> GAHMSGRGSSTDSMFSRFLPEKTDLKDYALPNASWCSDMLSLYQEFLEKTKSSGWIKLPSFKSNRDHIRGLKLPSGLAVSSDKGDCRIFTRCIQVEGQGFEYVIFFQPTQKKSVCLFQPGSYLEGPPGFAHGGSLAAMMDETFSKTAFLAGEGLFTLSLNIRFKNLIPVDSLVVMDVEVDKIEDQKLYMSCIAHSRDQQTVYAKSSGVFLQLQ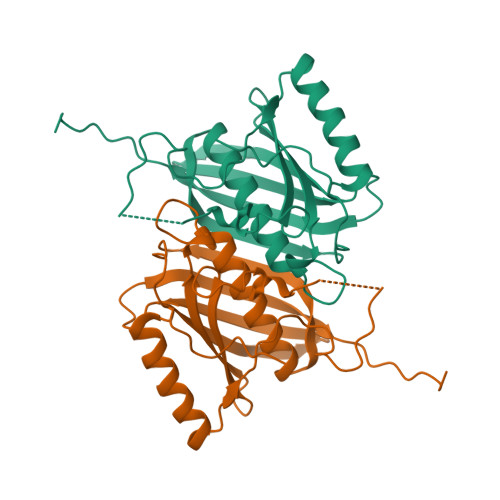LEEESPQ> GSMEKAAVNEDGLVIPLIDFSKFLEGDETLKLETAKAILHGFQTAGFIYLKNIPIQPDFREHVFNTSAKFFKLPKEKKLEVGWTTPEANRGYSAPGREKVTQLTDPAEIEKIRSAAPDIKESYEIGREDEPGHPNPWPAEQDDLVGFKSTMNNFFDQCKALHIEVMRAIAVGMGIDANYFDSFVDVGDNILRLLHYPAVKSEVFKINPGQVRAGEHTDYGS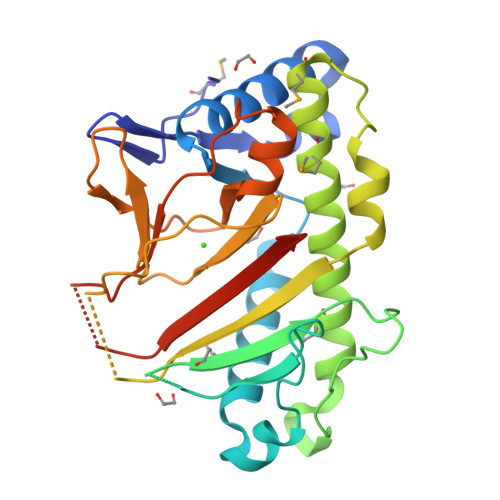ITLLFQDSRGGLQVKSPNGQFIDATPIENTVVVNAGDLLARWSNDTIKSTVHRVVEPPKQEDVHPPRYSIAYFCNPNHKSLEHHHHHH> PEGLEQLEAQTNFTKRELQVLYRGFKNECPSGVVNEDTFKQIYAQFFPHGDASTYAHYLFNAFDTTQTGSVKFEDFVTALSILLRGTVHEKLRWTFNLYDINKDGYINKEEMMDIVKAIYDMMGKYTYPVLKEDTPRQHVDVFFQKMDKNKDGIVTLDEFLESCQEDDNIMRSLQLFQNV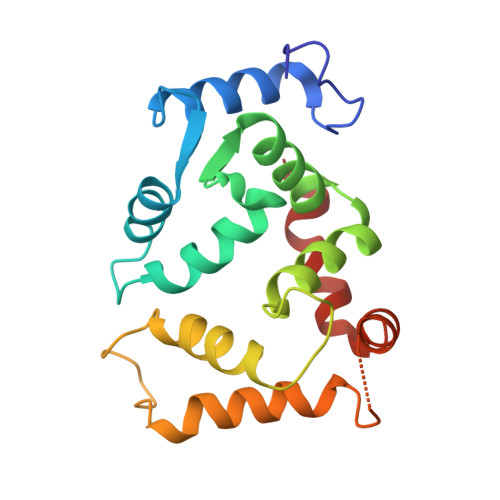M> SNADKPGEVADDGSVTVRHAFGDTTIPGPPQRVVSAGLTEQDDLLAVGVVPIAVTDWFGGEPFGVWPWAQRQLAGAQPAVLNLDNGIPVEEIAALKPDLIVATNAGLDADTYAKLSEIAPTVAQTGSEAFFEPWKDQATIIGQAVFKNAEMTELIKSVDDRFTTVKTDHPQFSGKKALLLGGTLYRGGVQATPPGWRTDFLTQMGLTVLQVPALIPRDEIASVLDGADVLIWTTESDQDRDALLADPIVAQLAATRRDRNIFTTKELAGAIAFASPLS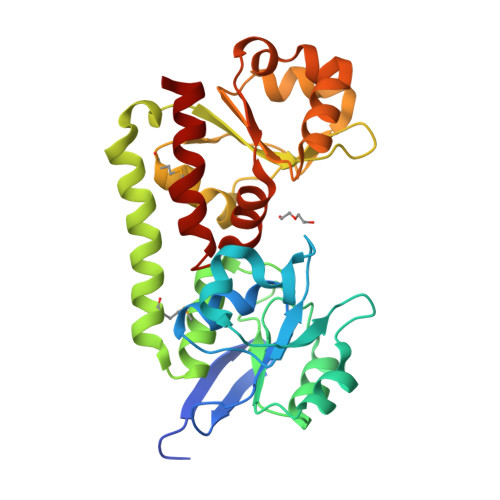YPVVADQLPPELARVLG>[12x]MVNSMFGGDLDPYEKSLNYEYPYHPSGNPKHIDVSEIDNLTLADYGWSPDAVKAYMFGIVVQNPDTGQPMGDEFYNHILERAVGKAERALDISILPDTQHEMRDYHETEFNSYMFVHAYRKPILQVENLQLQFNGRPIYKYPANWWKVEHLAGHVQLFPTALMQTGQSMSYDAVFNGYPQLAGVYPPSGATFAPQMIRLEYVSGMLPRKKAGRNKPWEMPPELEQLVIKYALKEIYQVWGNLIIGAGIANKTLEVDGITETIGTTQSAMYGGASAQILQINEDIKELLDGLRAYFGYNMIGL;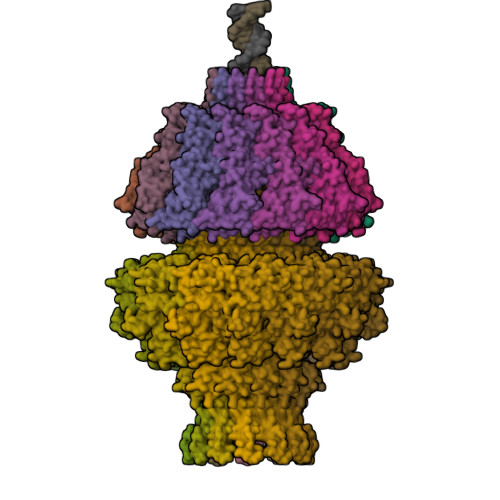>[12x]MADLFKQFRLGKDYGNNSTIAQVPIDEGLQANIKKIEQDNKEYQDLTKSLYGQQQAYAEPFIEMMDTNPEFRDKRSYMKNEHNLHDVLKKFGNNPILNAIILTRSNQVAMYCQPARYSEKGLGFEVRLRDLDAEPGRKEKEEMKRIEDFIVNTGKDKDVDRDSFQTFCKKIVRDTYIYDQVNFEKVFNKNNKTKLEKFIAVDPSTIFYATDKKGKIIKGGKRFVQVVDKRVVASFTSRELAMGIRNPRTELSSSGYGLSEVEIAMKEFIAYNNTESFNDRFFSHGGTTRGILQIRSDQQQSQHALENFKREWKSSLSGINGSWQIPVVMADDIKFVNMTPTANDMQFEKWLNYLINIISALYGIDPAEIGFPNRGGATGSKGGSTLNEADPGKKQQQSQNKGLQPLLRFIEDLVNRHIISEYGDKYTFQFVGGDTKSATDKLNILKLETQIFKTVNEAREEQGKKPIEGGDIILDASFLQGTAQLQQDKQYNDGKQKERLQMMMSLLEGDNDDSEEGQSTDSSNDDKEIGTDAQIKGDDNVYRTQTSNKGQGRKGEKSSDFKH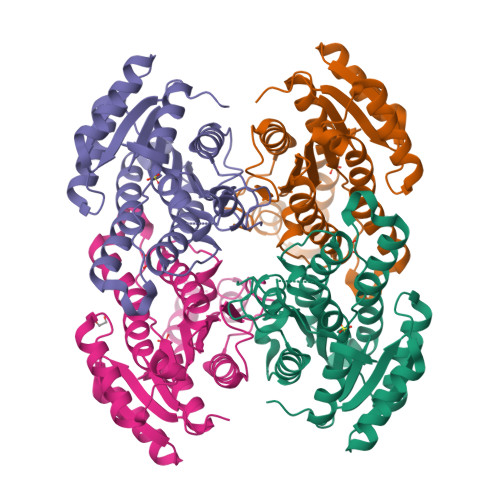>[8x]MAHHHHHHMSNLNGKTAVVTGAASGIGKEIALELAKAGAAVAIADLNQDGANAVADEINKAGGKAIGVAMDVTNEEAVNTGIDKVAEAFGSVDILVSNAGIQIVNPIENYSFADWKKMQAIHVDGAFLTTKAALKHMYKDDRGGVVIYMGSVHSHEASPLKSAYVTAKHGLLGLARVLAKEGAKHNVRSHVVCPGFVRTPLVDKQIPEQAKELGISEEEVIKKVMLGNTVDGVFTTVQDVAQTVLFLSAFPSAALTGQSFIVSHGWFMQ> MKTVNMKTGTDSFVGEDGKPETKDQYPWGLRITLDNESLQRLGL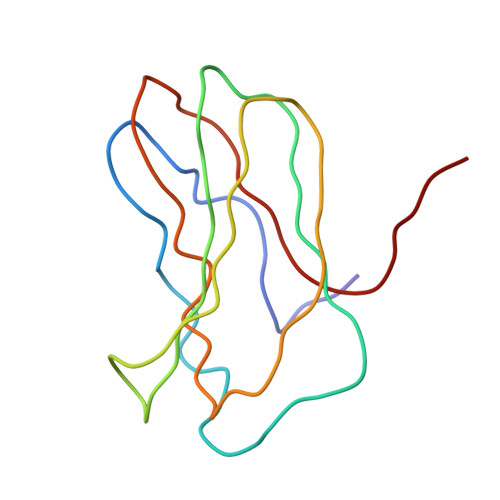NAKSLPAVGDSVSVMAMANVCSVSTRTTDHGEDNYVELQITDIGLAPQKRDDAKELKDAFYPDGEDD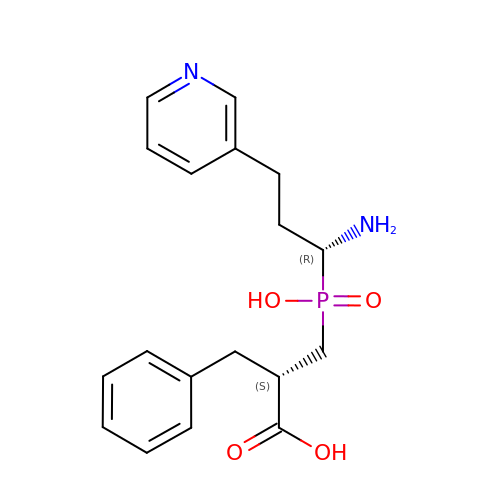3-{[(R)-1-amino-3-(pyridin-3-yl)propyl](hydroxy)phosphoryl}-(S)-2-benzylpropanoic acid | C18 H23 N2 O4 P | LWRKOPLMYMXZKW-IAGOWNOFSA-N> SPTVEECGYSDRVRSITLGNSTITTQECANVVVGYGRWPTYLRDDEATAEDQPTQPDVATCRFYTLDSIKWEKGSVGWWWKFPEALSDMGLFGQNMQYHYLGRAGYTIHVQCNASKFHQGCLLVVCVPEAEMGGAVVGQAF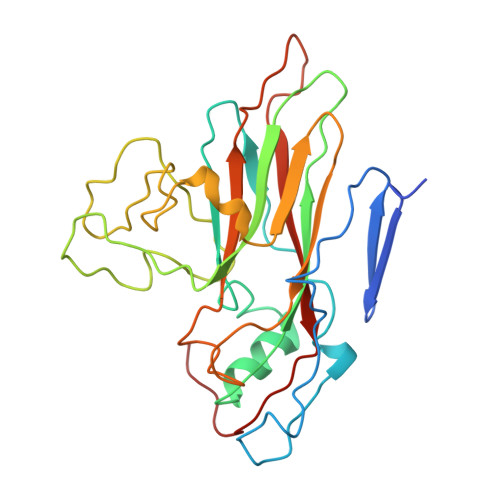SATAMANGDKAYEFTSATQSDQTKVQTAIHNAGMGVGVGNLTIYPHQWINLRTNNSATIVMPYINSVPMDNMFRHYNFTLMVIPFVKLDYADTASTYVPITVTVAPMCAEYNGLRLAQAQ> SYMVARMQKMKAGNLGGAFKHNERVFETHSNKDINPSRSHLNYELTDRDRSVSYEKQIKDYVNENKVSNRAIRKDAVLCDEWIITSDKDFFEKLDEEQTRTFFETAKNYFAENYGESNIAYASVHLDESTPHMHMGVVPFENGKLSSKAMFDREELKHIQEDLPRYMSDHGFELERGKLNSEAK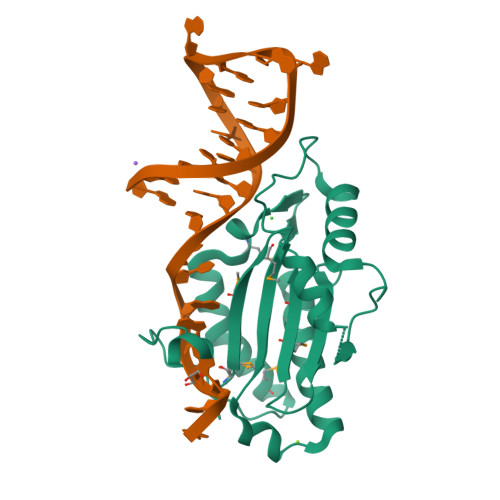HKTVAEFKRAMADM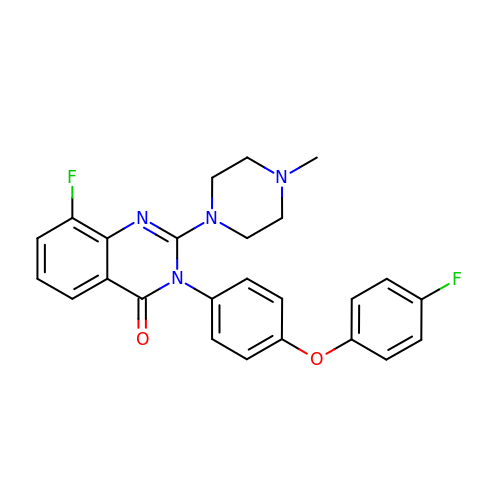8-fluoranyl-3-[4-(4-fluoranylphenoxy)phenyl]-2-(4-methylpiperazin-1-yl)quinazolin-4-one | C25 H22 F2 N4 O2 | NUGPMKZYSBKNPU-UHFFFAOYSA-N> MVSAIVLYVLLAAAAHSAFALQDPCSNCPAGTFCDNNRNQICSPCPPNSFSSAGGQRTCDICRQCKGVFRTRKECSSTSNAECDCTPGFHCLGAGCSMCEQD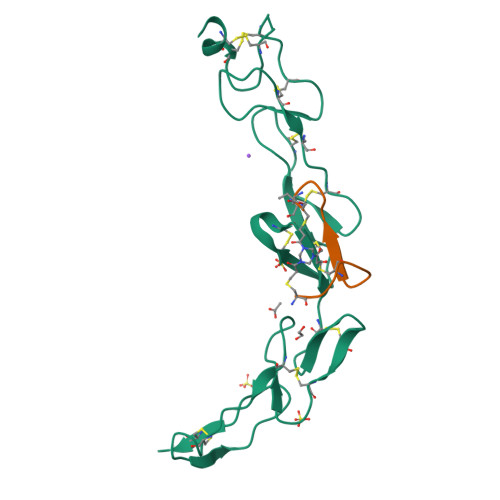CKQGQELTKKGCKDCSFGTFNDQKRGICRPWTDCSLDGKSVLVDGTKERDVVCGPGSHHHHHH;> CIEEGQYCFADPYLC>[2x]MDVNQQYNHFLKQHVDGEMTTLKCKSQMEILNL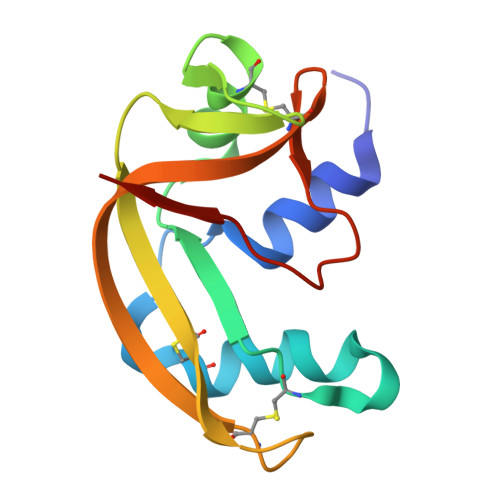NRPDRKCKLKNTFILANPDQVQAICTGGGTLKGNNLVQSNKPFSVVICTHTGGESHPNCTYKGSSATKKVIIACDGKFPVHYDGDVDIGITDGK> IEGYECQPIFLNVLEAIEPGVVCAGHDN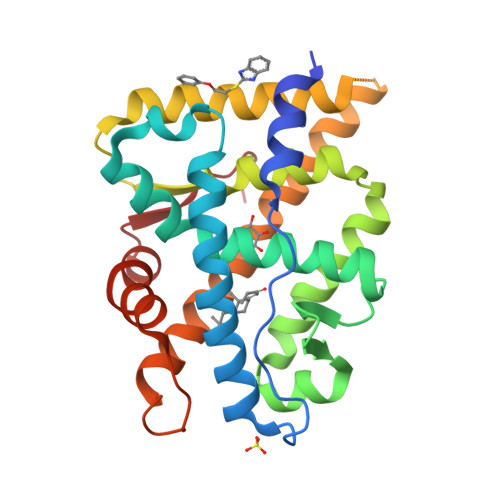NQPDSFAALLSSLNELGERQLVHVVKWAKALPGFRNLHVDDQMAVIQYSWMGLMVFAMGWRSFTNVNSRMLYFAPDLVFNEYRMHKSRMYSQCVRMRHLSQEFGWLQITPQEFLCMKALLLFSIIPVDGLKNQKFFDELRMNYIKELDRIIACKRKNPTSCSRRFYQLTKLLDSVQPIARELHQFTFDLLIKSHMVSVDFPEMMAEIISVQVPKILSGKVKPIYFHTQ>[4x]GKEWQENKSWNAHFSEHKTQGVVVLWNENTQQGFTNDLKRANQAFLPASTFKIPNSLIALDLGVVKDEHQVFKWDGQTRDIAAWN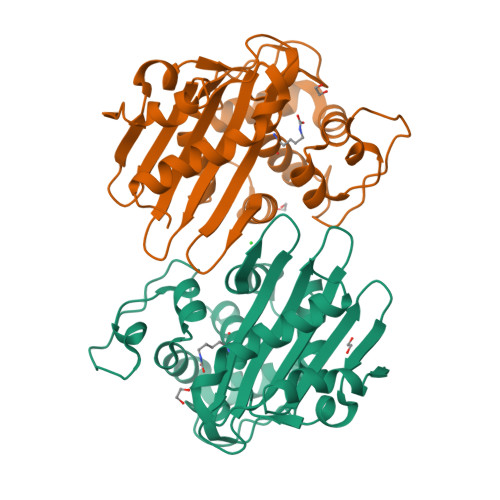RDHDLITAMKYSVVPVYQEFARQIGEARMSKMLHAFDYGNEDISGNLDSFWLDGGIRISATQQIAFLRKLYHNKLHVSERSQRIVKQAMLTEANADYIIRAKTGYSVRIEPKIGWWVGWIELDDNVWFFATNMDMPTAEGLGLRQTITKAVLKQEKIIP3'-DESAMINO-3'-(2-METHOXY-4-MORPHOLINYL)-DOXORUBICIN | 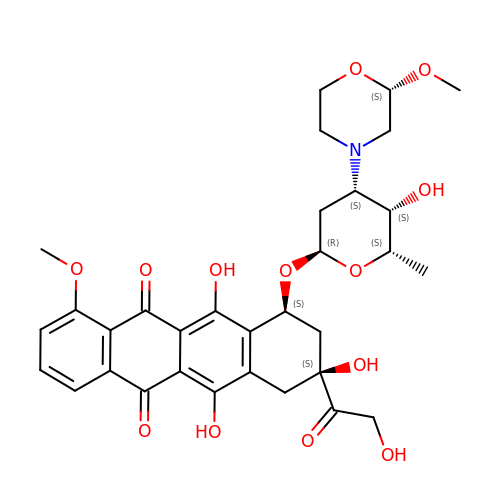C32 H37 N O13 | CTMCWCONSULRHO-UHQPFXKFSA-N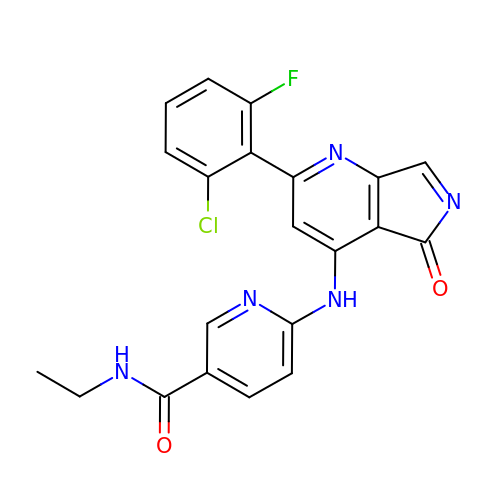6-{[(2M)-2-(2-chloro-6-fluorophenyl)-5-oxo-5H-pyrrolo[3,4-b]pyridin-4-yl]amino}-N-ethylpyridine-3-carboxamide | C21 H15 Cl F N5 O2 | GRSCUMLWKVMZMN-UHFFFAOYSA-N>MADSDINIKTGTTDIGSNTTVKTGDLVTYDKENGMAKKVFYSFIDDKNHNKKLLVIRTKGTIAGQYRVYSEEGANKSGLAWPSAFKVQLQLPDNEVAQISDYYPRNSIDTKEYMSTLTYGFNGNVTGDDTGKIGGLIGANVSIGHTLKYVQPDFKTILESPTDKKVGWKVIFNNMVNQNWGPYDRDSWNPVYGNQLFMKTRNGSMKAAENFLD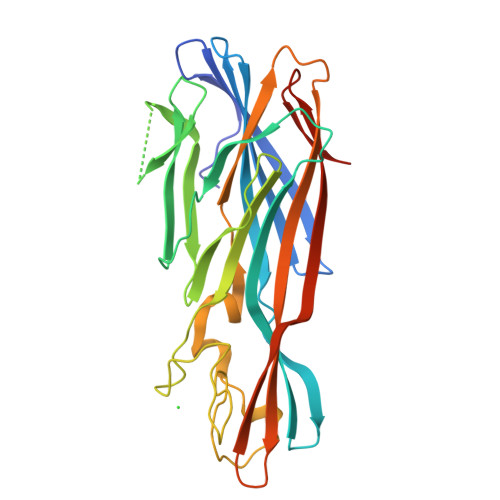PNKASSLLSSGFSPDFATVITMDRKASKQQTNIDVIYERVRDDYQLHWTSTNWKGTNTKDKWTDRSSERYKIDWEKEEMTNLEHHHHHH[6x]>[4x]MAHHHHHHMKVGLVGWRGMVGSVLMQRMVEENDFAHIEPFYFSTSNAGGEAPSFGGKTAPALMEATDITSLKQMDVIITCQGGDYTSEVFPKLKATGWDGYWIDAASTLRMTDDAIIVLDPVNLNVIKDGLAKGTKTF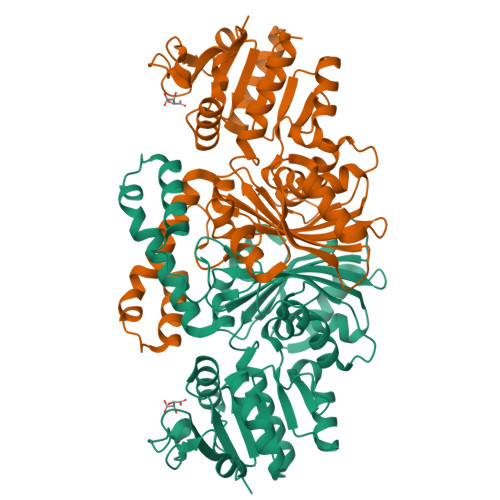VGGNCTVSLMLMGVGALFQNNLVEWMTAMTYQAASGAGAQNMRELLTGMGYLYNNTKTLLDDPKSAILDIDRQVAELQRGEGFPSANFGVPLAGSLIPYIDKQLESGQSKEEWKGQVETNKILGNSQIVPIDGHCVRIGAMRCHSQALTIKLKKDVPLDEIEDMIRNSNQWAKVVPNTREASMTDLTPVAVTGTLTVPVGRLRKLNMGKEYLGAFTVGDQLLWGAAEPLRRMLRILVEYKSS>MHHHHHHSSGRENLYFQGMKLKEVDRTAMQAWSPAQNHPIYLATGTSAQQLDATFSTNASLEIFELDLSDPSLDMKSCATFSSSHRYHKLIWGPYKMDSKGDVSGVLIAGGENGNIILYDPSKIIAGDKEVVIAQNDKHTGPVRALDVNIFQTNLVASGANESEIYIWDLNNFATPMTPGAKTQPPEDISCIAWNRQVQHILASASPSGRATVWDLRKNEPIIKVSDHSNRMHCSGLAWHPDVATQMVLASEDDRLPVIQMWDLRFASSPLRVLENHARGILAIAWSMADPELLLSCGKDAKILCSNPNTGEVL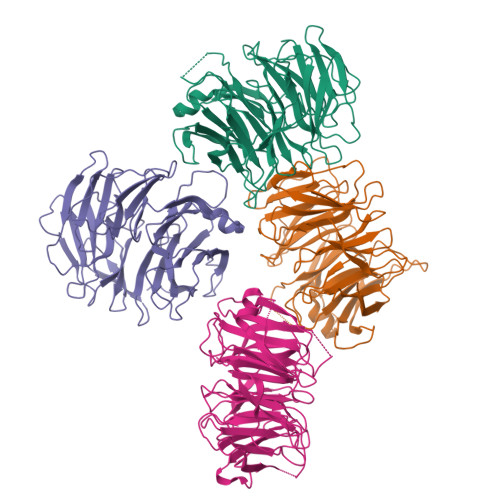YELPTNTQWCFDIQWCPRNPAVLSAASFDGRISVYSIMGGST[4x]> MAANNNPQGTKPNSLVCANCEGEGCVACSQCKGGGVNLIDH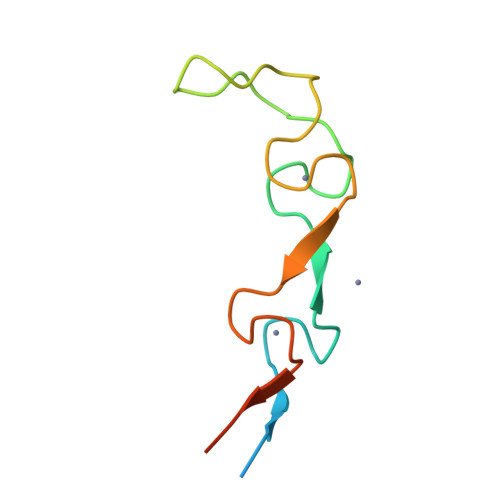FNGQFKAGALCWLCRGKKEVLCGDCNGAGFIGGFLSTFDE>[2x]MPYIEKLELKGF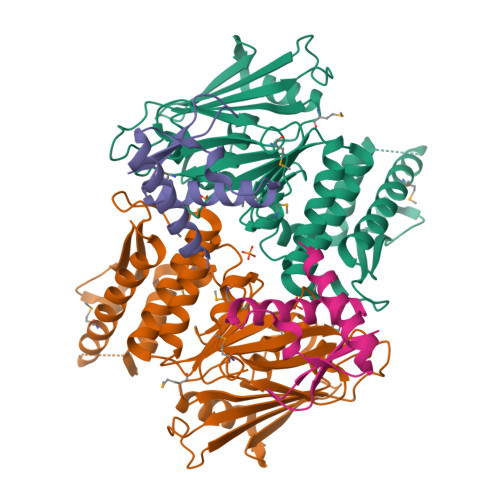KSYGNKKVVIPFSKGFTAIVGANGSGKSNIGDAILFVLGGLSAKAMRASRISDLIFAGSKNEPPAKYAEVAIYFNNEDRGFPIDEDEVVIRRRVYPDGRSSYWLNGRRATRSEILDILTAAMISPDGYNIVLQGDITKFIKMSPLERRLLIDDISGIAEYDSKKEKALEEEKEKKNVFMRTFEAISRNFSEIFAKLSPGGSARLILENPEDPFSGGLEIEAKPAGKDVKRIEAMSGGEKALTALAFVFAIQKFKPAPFYLFDEIDAHLDDANVKRVADLIKESSKESQFIVITLRDVMMANADKIIGVSMRDGVSKVVSLSLEKAMKILEEIRKKQGWEHGN;>[2x]KKVEIDEEIFVIDDFRVDIEKYVEELYKVVKKIYEKTGTPIKFWDLVPDVEPKIIARTFLYLLFLENMGRVEIIQEEPFGEILVVPM[N-(BENZYLOXYCARBONYL)AMINO](4-AMIDINOPHENYL)METHANE-PHOSPHONATE | C16 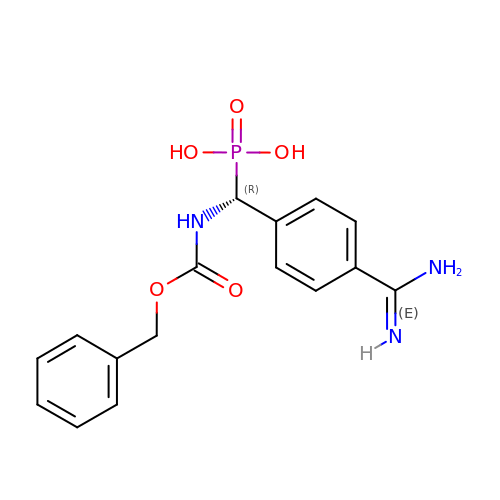H18 N3 O5 P | FSNDLCSOLUMYRH-OAHLLOKOSA-N> TTFADLGLKAPILEALNDLGYEKPSPIQAECIPHLLNGRDVLGMAQTGSGKTAAFSLPLLQNLDPELKAPQILVLAPTRELAVQVAEAMTDFSKHMRGVNVVALYGGQRYDV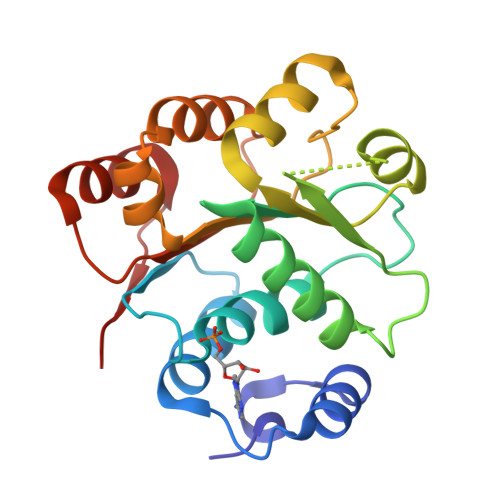QLRALRQGPQIVVGTPGRLLDHLKRGTLDLSKLSGLVLDEADEMLRMGFIEDVETIMAQIPEGHQTALFSATMPEAIRRITRRFMKEPQEVRI>MGSMTVQEDDKRTSDESMSIDNLRGFVDLNVGKWTGSFHQFDGNGNLLHKIDTRLSASSYGEDELLSLNQSLYIKQPTSATSVSEEEEE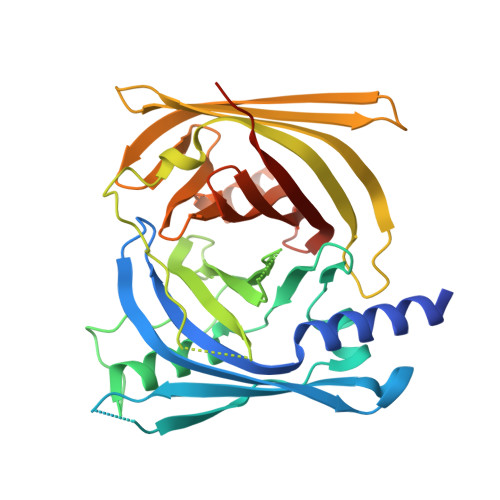EPEWVEYKIKETNMFTVDKYQQIGFFPKERAFSLRYQTAGMLDTTLRQGVLGEDDTGEESPRNLKLPSRRPSLVCENCLYSKEIDRRARAFHIMDPKGVLEMLIVFLEERGLENLAHPVLDNAQNDAERINPFLGTWKGRSVTKRSGVYGATLSEADTVAVLEMNDKGQVVQDISSTSDEKKVTTNVHWEGKMSKDLVTFAEGYQMTLLPGGMYMGCPCDVSKCVADLKSFHLEFCWLESPSSRQRLIRTYDHEGLAVSSTYFTETKMKLAAALEHHHHHH[4x]> UUCCAGUGCGGAGUCUGGAGACACCCAGGGGGAAGCGAAGACCCUAUGGAGCUUUACUGCAGGCUGUCGCUGAGACGUGGUCGCCGAUGUGCAGCAUAGGUAGGAGACACUACACAGGUACCCGCGCUAGCGGGCCACCGAGUCAACAGUGAAAUACUACCCGUCGGUGACUGCGACUCU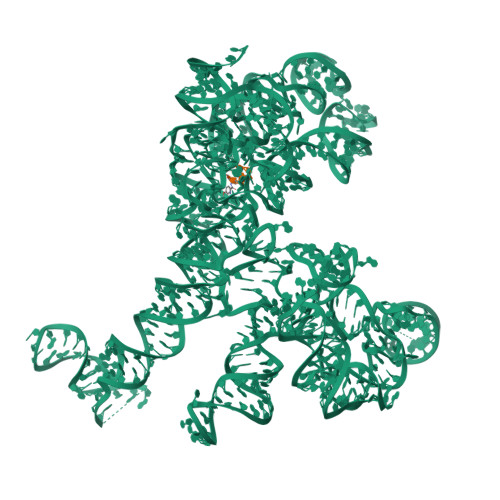CACUCCGGGAGGAGGACACCGAUAGCCGGGCAGUUUGACUGGGGCGGUACGCGCUCGAAAAGAUAUCGAGCGCGCCCUAUGGCUAUCUCAGCCGGGACAGAGACCCGGCGAAGAGUGCAAGAGCAAAAGAUAGCUUGACAGUGUUCUUCCCAACGAGGAACGCUGACGCGAAAGCGUGGUCUAGCGAACCAAUUAGCCUGCUUGAUGCGGGCAAUUGAUGACAGAAAAGCUACCCUAGGGAUAACAGAGUCGUCACUCGCAAGAGCACAUAUCGACCGAGUGGCUUGCUACCUCGAUGUCGGUUCCCUCCAUCCUGCCCGUGCAGAAGCGGGCAAGGGUGAGGUUGUUCGCCUAUUAAAGGAGGUCGUGAGCUGGGUUUAGACCGUCGUGAGACAGGUCGGCUGCUAUCUACUGGGUGUGUA;> CCGGCGGGCUGGUUCAAACCGGCCCGCCGGACCA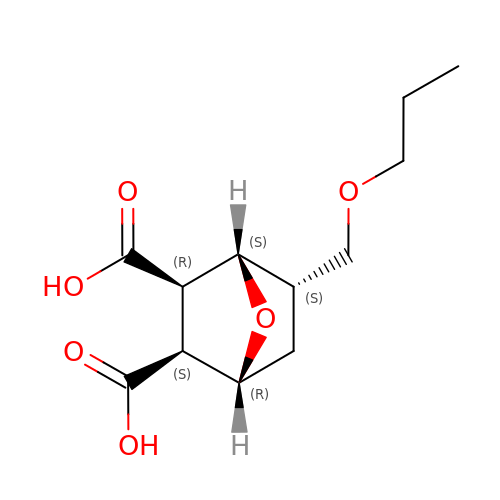(1R,2S,3R,4S,5S)-5-(propoxymethyl)-7-oxabicyclo[2.2.1]heptane-2,3-dicarboxylic acid | C12 H18 O6 | KENGHAXMPKBHLS-CHHOWFRJSA-N One such an example is glutamine synthetases (GSs) (EC 6.3.1.2), one of the most ancient functioning enzymes in existence and a central enzyme in nitrogen metabolism of all living organisms, catalyzing the formation of glutamine by condensation of glutamate with ammonia using ATP as an energy source. Decades of studies have established a striking notion that all three classes of GS enzymes, despite of dramatic differences in amino acid sequences and protein sizes, share quaternary geometry in dihedral symmetry assembled with two oligomeric rings. Considering that the active sites of GS are located at the clefts formed between two neighboring protomers within the same ring and distal to the ring-ring interface, each isolated GS subcomplex ring holds multiple integral catalytic sites. Cryo-EM structure determination of GS in both the catalytically active and inactive assembly states allows us to reveal an unanticipated self-assembly-induced disorder-order transition paradigm, in which the remote interactions between two subcomplex entities significantly rigidify the otherwise structurally fluctuating active sites, thereby regulating activity.

In order to elucidate the mechanism of how the pentameric CsGSIb (thereafter named as CsGSIbPen) demonstrates distinct enzymatic properties than CsGSIbDec, we next determined the structure of CsGSIbPen. Lowering the sample concentration, which favored pentamer dissociation, allowed us to obtain sufficient number of CsGSIbPen particles (Figure 3—figure supplements 2 and 3), which, in turn, enabled us to solve the cryo-EM structure of the inactive single-ringed GSII for the first time. Unexpected, CsGSIbPen exhibited high conformational heterogeneity and 3D particles classification generated three similar structures with the r.m.s.d. ranging from 0.6 to 0.8 Å, differing in a few peripheral regions. The most striking difference between CsGSIbPen and CsGSIbDec is that several regions are missing in the electron density map of all three classifications of CsGSIbPen particles, with only 229–255 out of 356 residues electron densities in presence. As a result, CsGSIbPen demonstrated a decagram-shaped density map with a few regions missing at the rim, in sharp contrast to a pentagon-shaped map yielded by the CsGSIbDec particles. For the 229–255 residues that show clear density in CsGSIbPen particles, the conformation of each subunit in three CsGSIbPen EM structures, as well as the arrangement pattern, closely resembles that of the CsGSIbDec, as evidenced by r.m.s.d. in the range of 0.7–1.0 Å. The density-missing regions include the segments around residues of 110–117, 140–166, and 260–334, among which, the fragment around residues 260–334 is a major component making up an integral catalytic site, while the segment of residues 140–166 comprising of the two gear teeth is responsible for ring-ring interaction (–4d).

>MSLLSDLCNLNLSESTEKIIAEYIWIGGSGMDLRSKARTLNAPVSDPSKLPQWNYDGSSTGQAPGEDSEVILYPQAIYKDPFRRGNNILVMCDAYTPGGEPIPTNKRFDAAKIFSHPDVVAEEPWYGIEQEYTLLQKEVKWPIGWPVGGYPGPQGPYYCGIGADKAFGRDIVDAHYKACLYAGINISGINGEVMPGQWEFQVGPSVGISSGDQLWMARYILERITEIAGVVVSFDPKPIEGDWNGAGAHTNYSTKSMRSDGGFEVIKKAIEKLGLKHREHIAAYGEGNERRLTGKHETADINTFLWGVANRGASIRVGRDTEKAGKGYFEDRRPASNMDPYIVTSMIANTTILWKP[5x]> MTMVGLIWAQATSGVIGRGGDIPWRLPEDQAHFREITMGHTIVMGRRTWDSLPAKVRPLPGRRNVVLSRQADFMASGAEVVGSLEEALTSPETWVIGGGQVYALALPYATRCEVTEVDIG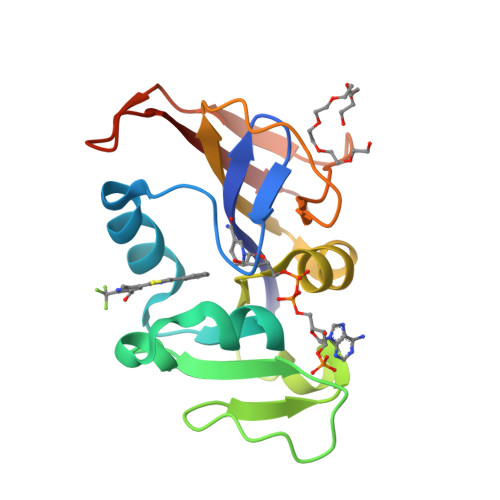LPREAGDALAPVLDETWRGETGEWRFSRSGLRYRLYSYHRS> ETSPLET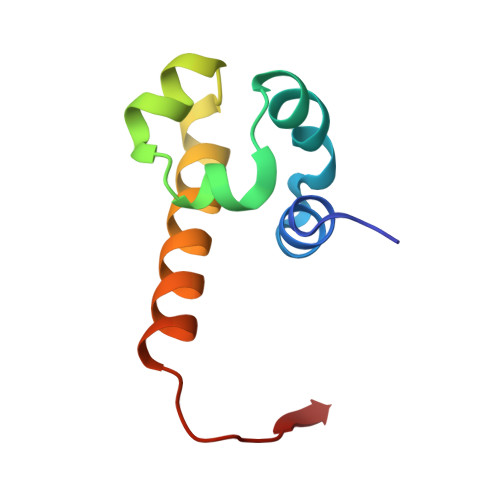FLASLHMEDFAALLRQEKIDLEALMLCSDLDLRSISVPLGPREKILGAVRRRRQAMERPPALEDTEL(4S,8aS)-hexahydroimidazo[1,5-a]pyridin-3(2H)-one 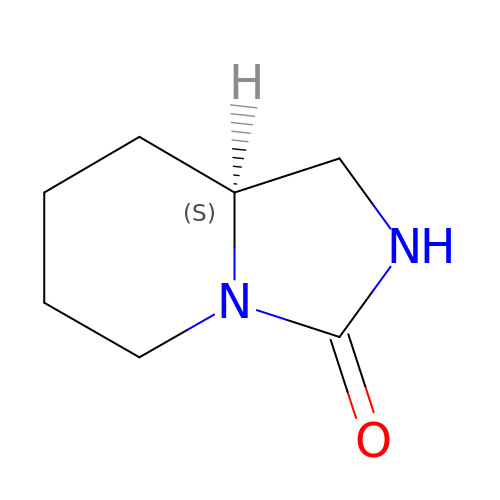| C7 H12 N2 O | QIWVINXQBDDSBJ-LURJTMIESA-N>MSLDDKATKPHDRLAQALAEDMAAVNALIRERMSSEHAPRIPEVTAHLIEAGGKRLRPMLTLAAARLVGYGGPFHVHLAATVEFIHTATLLHDDVVDESRQRRGRPTANLLWDNKSSVLVGDYLFARSFQLMTDTGNMRVMEILANASAVIAEGEVLQLTAAQNLATTEDIYLRVIRGKTAALFSAATEVGGIIGGAPEDQVQALFDYGDALGIAFQIVDDLLDYGGKSAEIGKNTGDDFRERKLTMPVIKAVALADEAERAFWKRVIEKGDQQDGDLEHAMALMTKHGTLEATRLAAIGWTDT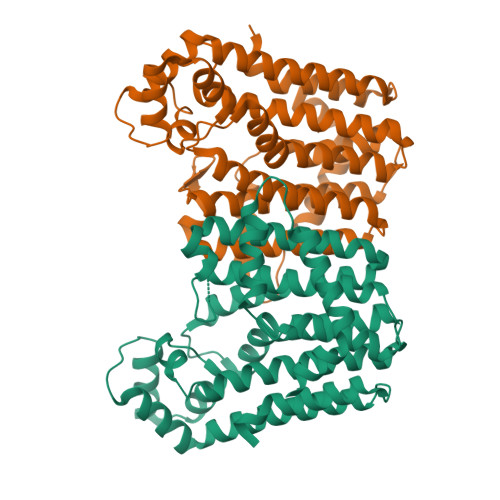ARKALAKLPDHPLRQMLDDLADYVVERVREGHHHHHH[2x]~{N}-[2,4-bis(fluoranyl)-3-[4-[3-[(3~{S})-1-propanoylpyrrolidin-3-yl]oxy-1~{H}-pyrazolo[3,4-b]pyridin-5-yl]-1,2,3-triazol-1-yl]phenyl]-3-phenyl-benzenesulfonamide 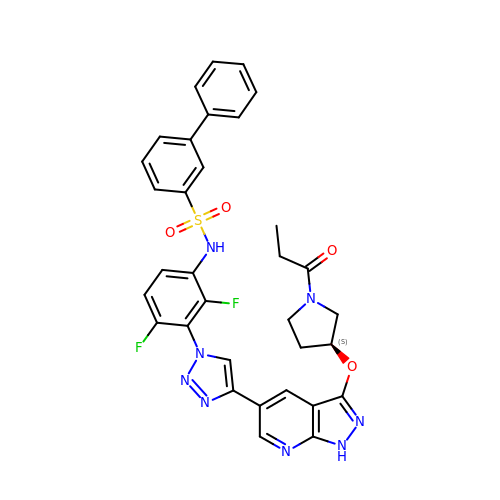| C33 H28 F2 N8 O4 S | MKXHLTDMQUDXEC-QHCPKHFHSA-N>MASGTDTGRFSRNLKDRLESNNYEEMELPPPTKGVIIPVVHTVESAPGEAFGSLLVIIPGAYPELLDPNQQVLSHFKNDTGCVWGIGEDIPFEGDDICYTALPLKEIKKDGNIVVEKVFAGPAMGPSCQLGLSLLVNDIDKGVPRMVFTGEIANDEETIVPICGVDIKAIAAHEHGLPLV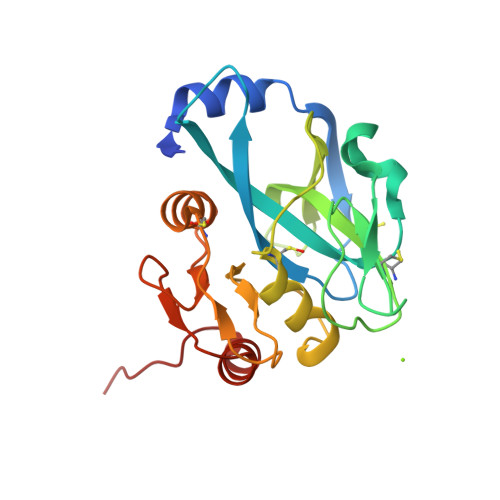GCQPGVDEVVANTSLASHLIQSGALPVQKA[5x]>MVSDAHFQGQFEVELKYRVKNHDAFLNMVKQIEHEVMFENNQESDWFYDTPQRTLTQQGKSLVLREIQPAGIKLWIVKGPEADRCEATNITKLDSAQSMLENMGYEVIQCSKKIRSIFFVGEFHITLDFLDGFGHFAEFAIMTDDETALARYRERLVALAQ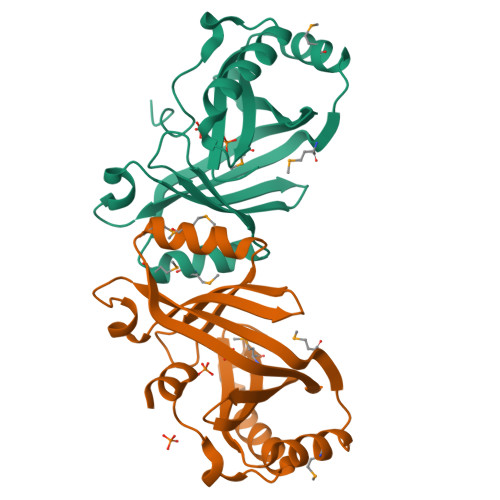QFHLSEADREHRSYKEILSALEHHHHHH[2x]Here we report the mechanism of three Fe(II)/α-ketoglutarate-dependent dioxygenases in bicyclomycin synthesis, which depicts the natural tactic to sequentially hydroxylate specific C−H bonds of similar substrates (cyclodipeptides). Three αKGDs (BcmE/BcmC/BcmG) catalyze site- and stereo-selective hydroxylation of inert C−H bonds in BCM’s (bicyclomycin) cyclic dipeptide scaffold (Fig. 1b3), one of the simplest peptide derivatives without additional functional groups. Our hypothesis posits distinct regulatory mechanisms: BcmE employs steric hindrance, BcmC relies on inherent reactivity, while BcmG utilizes a directing group to control C–H hydroxylation. Although these three enzymes share only 35–42% amino acid identities, the overall structures are similar, and r.m.s.d. values are 0.70 Å (SsBcmE vs SsBcmC), 1.07 Å (SsBcmE vs PaBcmG) and 0.87 Å (SsBcmC vs PaBcmG), respectively.

We subsequently selected the homologous enzymes and finally obtained the crystals of the ternary complexes of PaBcmG (from Pseudomonas aeruginosa), which also catalyzed the conversion of substrate 3 to 4. As a result, we determined a collection of X-ray crystal structures including ternary complexes of SsBcmE, SsBcmC, PaBcmG (with Fe(II) or/and αKG). Likewise, the comparison between PaBcmG•FeII•αKG and PaBcmG•FeII•αKG•3 structures revealed that the C-terminal helix may function as a gate or lid for the active pocket, and the binding of substrate triggers the closure of this gate.

>[4x]MNPNATYALASAELIDGKLRFDSSDGFARAIADGFFFVKSPSLDLAAGDTFARNFYLPRQEGLGAPYQGFSQWTEDRLARREGYFSRDVDQVEQFFLESRFWQTVFPGPLLRQAERMRSFSLEVLRAVLAELDLPVELWDEATGRCLSMQGTYHLTFNHFRSHVRARGLNVHKDSGWVTILRSLEPGLEVLREGDWLPVSPRPGEFIVNFGCAMEILTRHSATPVAAVAHRVQEQLPGQADRFSYALFVDSSLDPRTCPGLFRYLPGHGLVLEADFEMFLNEILHNTYQENTQGLYLEHHHHHHHH>MRKFRLIPYKQVDKVSALSEVPMGVEIVEAPAVWRASAKGAGQIIGVIDTGCQVDHPDLAERIIGGVNLTTDYGGDETNFSDNNGHGTHVAGTVAAAETGSGVVGVAPKADLFIIKALSGDGSGEMGWIAKAIRYAVDWRGPKGEQMRIITMSLGGPTDSEELHDAVKYAVSNNVSVVCAAGNEGDGREDTNEFAYPAAYNEVIAVGAVDFDLRLSDFTNTNEEIDIVAPGVGIKSTYLDSGYAELSGTAMAAPHVAGALALIIN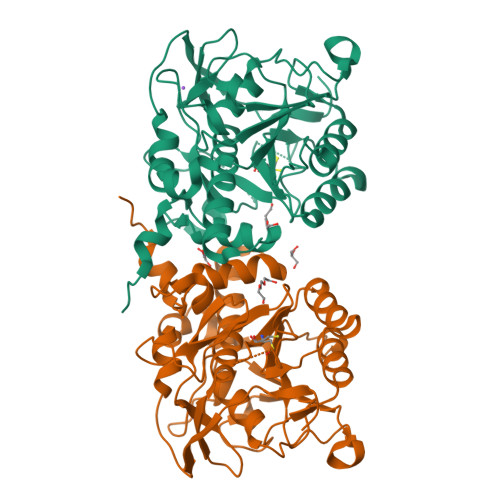LAEDAFKRSLSETEIYAQLVRRATPIGFTAQAEGNGFLTLDLVERITGQFTEKGKKHHHHHH[6x]> MSEPRFVHLRVHSDYSMIDGLAKTAPLVKKAAALGMPALAITDFTNLCGLVKFYGAGHGAGIKPIVGADFNVQCDLLGDELTHLTVLAANNTGYQNLTLLISKAYQRGYGAAGPIIDRDWLIELNEGLILLSGGRMGDVGRSLLRGNSALVDECVAFYEEHFPDRYFLELIRTGRPDEESYLHAAVELAEARGLPVVATNDVRFIDSSDFDAHEIRVAIHDGFTLDDPKRPRNYSPQQYMRSEEEMCELFADIPEALANTVEIAKRCNVTVRLGEYFLPQFPTGDMSTEDYLVKRAKEGLEERLAFLFPDEEERLKRRPEYDERLETELQVINQMGFPGYFLIVMEFIQWSKDNGVPVGPGRGSGAGSLVAYALKITDLDPLEFDLLFERFLNPERVSMPDFDVDFCMEKRDQVIEHVADMYGRDAVSQIITFGTMAAKAVIRDVGRVLGHPYGFVDRISKLIPPDPGMTLAKAFEAEPQLPEIYEADEEVKALIDMARKLEGVTRNAGKHAGGVVIAPTKITDFAPLYCDEEGKHPVTQFDKSDVEYAGLVKFDFLGLRTLTIINWALEMINKRRAKNGEPPLDIAAIPLDDKKSFDMLQRSETTAVFQLESRGMKDLIKRLQPDCFEDMIALVALFRPGPLQSGMVDNFID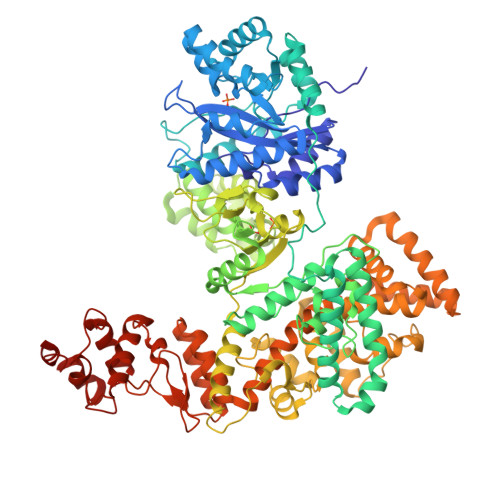RKHGREEISYPDVQWQHESLKPVLEPTYGIILYQEQVMQIAQVLSGYTLGGADMLRRAMGKKKPEEMAKQRSVFAEGAEKNGINAELAMKIFDLVEKFAGYGFNKSHSAAYALVSYQTLWLKAHYPAEFMAAVMTADMDNTEKVVGLVDECWRMGLKILPPDINSGLYHFHVNDDGEIVYGIGAIKGVGEGPIEAIIEARNKGGYFRELFDLCARTDTKKLNRRVLEKLIMSGAFDRLGPHRAALMNSLGDALKAAD>LPDSVDWREKGCVTEVKYQGSCGACWAFSAVGALEAQLKLKTGKLVSLSAQNLVDCSTEKYGNKGCNGGFMTTAFQYIIDNKGIDSDASYPYKAMDQKCQYDSKYRAATCSKYTELPYGREDVLKEAVANKGPVSVGVDARHPSFFLYRSGVYYEPSCTQNVNHGVLVVGYGDLNGKEYWLVKNSWGHNF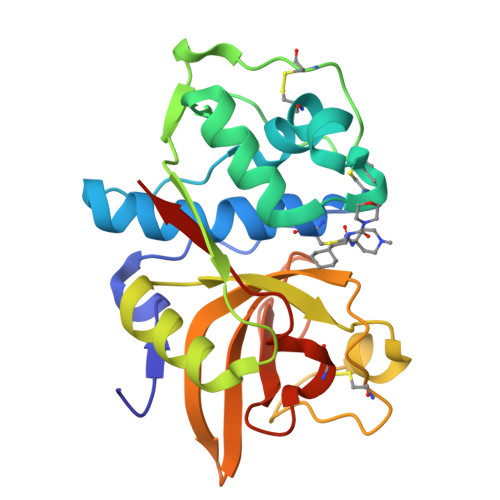GEEGYIRMARNKGNHCGIASFPSYPEIHHHHH[2x]> AVPSTQTPWGIKSIYNDQSITKTTGGSGIKVAVLDTGVYTSHLDLAGSAEQCKDFTQSNPLVDGSCTDRQGHGTHVAGTVLAHGGSNGQGVYGVAPQAKLWAYKVLGDNGSGYSDDIAAAIRHVADEASRTGSKVVINMSLGSSAKDSLIASAVDYAYGKGVLIVAAAGNSGSGSNTIGFPGGLVNAVAVAALENVQQNGTYRVADFSSRGNPATAGDYIIQERDIEVSAPGASVESTWYTGGYNTISGTSMATPHVAGLAAKIWSANTSLSHSQLRTELQNRAKVYD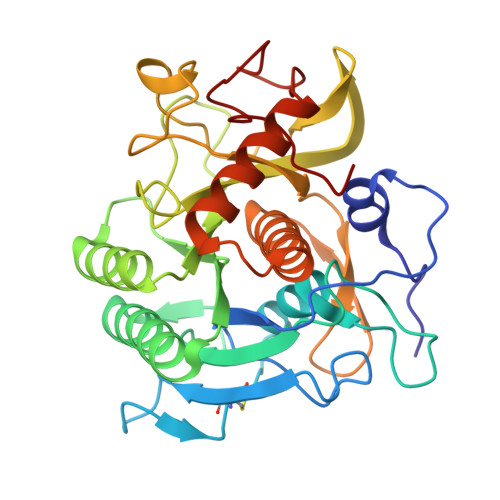IKGGIGAGTGDDYASGFGYPRVK> MGSDKIHHHHHHMSAIERITKAAHLIDMNDIIREGNPTLRTVAEEVTFPLSDQEIILGEKMMQFLKHSQDPVMAEKMGLRGGVGLAAPQLDISKRIIAVLVPNIVEEGETPQEAYDL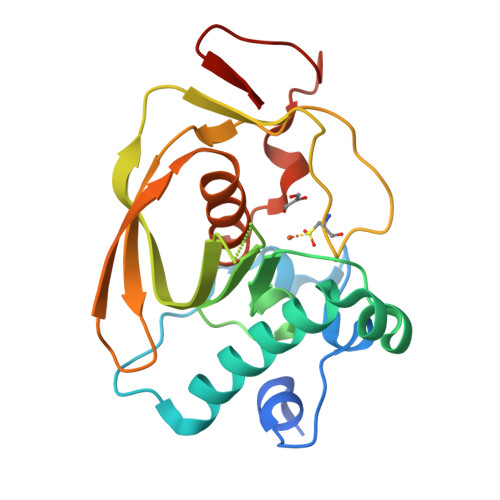EAIMYNPKIVSHSVQDAALGEGEGCLSVDRNVPGYVVRHARVTVDYFDKDGEKHRIKLKGYNSIVVQHEIDHINGIMFYDRINEKDPFAVKDGLLILE>MSTEHVDHKTIARFAEDKVNLPKVKADDFREQAKRLQNKLEGYLSDHPDFSLKRMIPSGSLAKGTALRSLNDIDVAVYISGSDAPQDLRGLLDYLADRLRKAFPNFSPDQVKPQTYSVTVSFRGSGLDVDIVPVLYSGLPDWRGHLISQEDGSFLETSIPLHLDFIKARKRAAPKHFAQVVRLAKYWARLMKQERPNFRFKSFMIELILAKLLDNGVDFSNYPEALQAFFSYLVSTELRERIVFEDNYPASKIGTLSDLVQIIDPVNPVNNVARLYTQSNVDAIIDAAMDAGDAIDAAFYAPTKQLTVTYWQKVFGSSFQG[2x];>[2x]MKSSHHHHHHENLYFQSNATFSVTHARHMAAK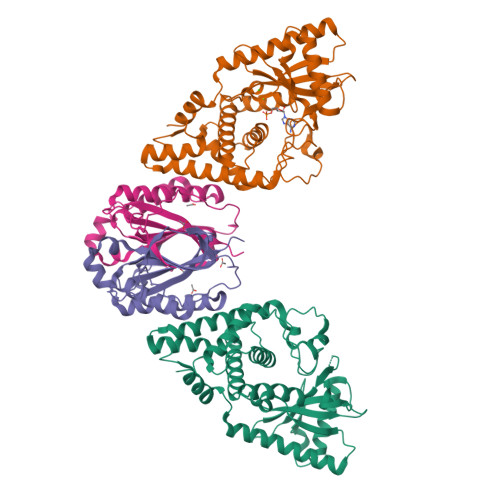VATDLRRMQRFYGYPSDADIEAYEEELVVFLKAGYLGEVSYGFQKNNNWIEPTLRYTAGDLLGSGTDDDPGKIRPGKDVSGASFYSFMTYSSKYLNATQSEKDTALKDLPFKRVGAQSPGINGYLENDKTYSAGGRSLTRTSVRNFV2-[(2-carboxyphenyl)amino]-5-(4-phosphonobutoxy)benzoic acid | C18 H20 N O8 P | 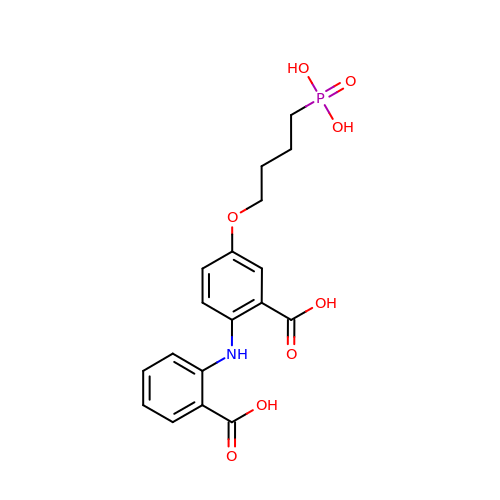VJUHVFNGPLDDFZ-UHFFFAOYSA-N>[8x]MKTVNVPSNGREKF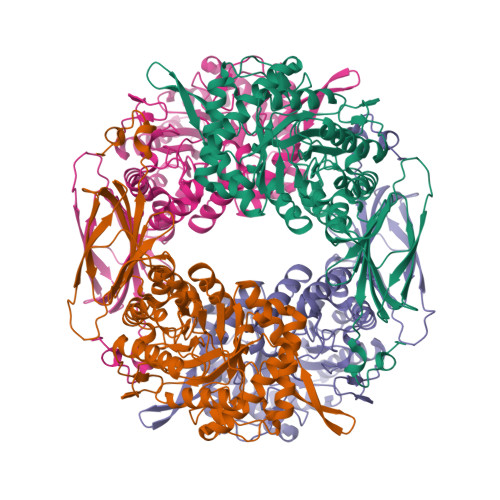KKNWKFCVGTGRLGLALQKEYLDHLKLVQEKIGFRYIRGHGLLSDDVGIYREVEIDGEMKPFYNFTYIDRIVDSYLALNIRPFIEFGFMPKALASGDQTVFYWKGNVTPPKDYNKWRDLIVAVVSHFIERYGIEEVRTWLFEVWNEPNLVNFWKDANKQEYFKLYEVTARAVKSVDPHLQVGGPAICGGSDEWITDFLHFCAERRVPVDFVSRHAYTSKAPHKKTFEYYYQELEPPEDMLEQFKTVRALIRQSPFPHLPLHITEYNTSYSPINPVHDTALNAAYIARILSEGGDYVDSFSYWTFSDVFEEMDVPKALFHGGFGLVALHSIPKPTFHAFTFFNALGDELLYRDGEMIVTRRKDGSIAAVLWNLVMEKGEGLTKEVQLVIPVSFSAVFIKRQIVNEQYGNAWRVWKQMGRPRFPSRQAVETLRQVAQPHVMTEQRRATDGVIHLSIVLSKNEVTLIEIEQVRDETSTYVGLDDGEITSYSS> 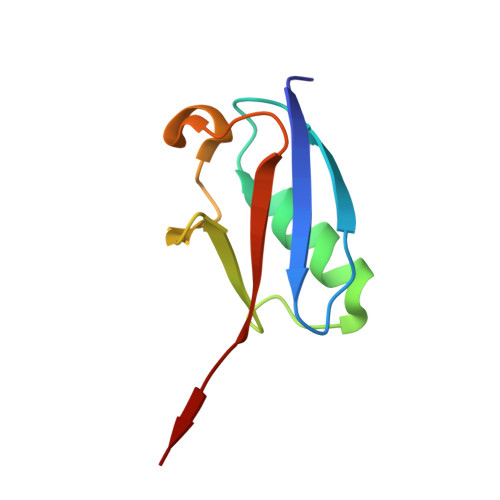EYIKLKVIGQDSSEIHFKVKMTTHLKKLMESYCQRQGVPMNSLRFLWEGQRIADNHTPKELGMEEEDVIEVYQEQTGG>[2x]GPEKIRPECFELLRVLGKGGYGKVFQVRKVTGANTGKIFAMKVLKKAMIVRNAKDTAH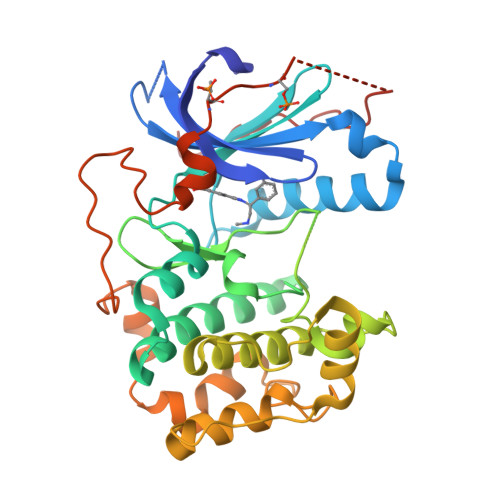TKAERNILEEVKHPFIVDLIYAFQTGGKLYLILEYLSGGELFMQLEREGIFMEDTACFYLAEISMALGHLHQKGIIYRDLKPENIMLNHQGHVKLTDFGLCKESIHDGTVTHTFCGTIEYMAPEILMRSGHNRAVDWWSLGALMYDMLTGAPPFTGENRKKTIDKILKCKLNLPPYLTQEARDLLKKLLKRNAASRLGAGPGDAGEVQAHPFFRHINWEELLARKVEPPFKPLLQSEEDVSQFDSKFTRQTPVDSPDDSTLSESANQVFLGFEYVAPSVLES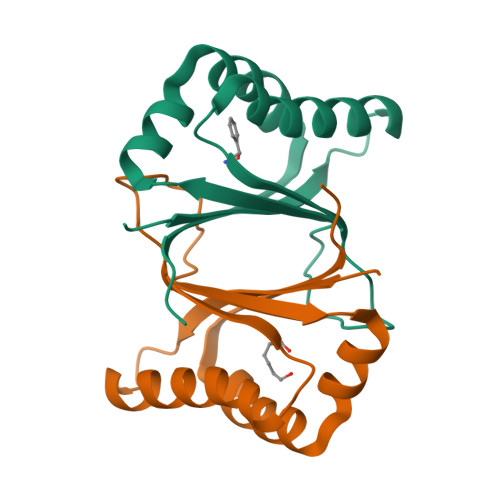>[12x]GNPPEIVRHIVFNRYKSQLSQKQIDQIIADYGNLQNIAPEMKEWKWGTDLGPAVEDRADGFTHAYESTFHSVADFLNFFYSPPALEFAKEFFPACEKIVVLNYIINE> SAPSVKGVSFDQANNLLIEPARIEEEELTLTILRQTGGLGISIAGGKGSTPYKGDDEGIFISRVSEEGPAARAGVRVGDKLLEVNGVALQGAEHHEAVEAL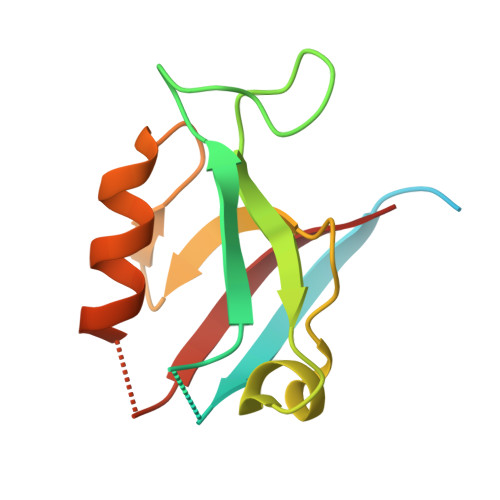RGAGTAVQMRVWRERM>MGSDKIHHHHHHENLYFQGMKQIPQDFRLIEDFFRTRRSVRKFIDRPVEEEKLMAILEAGRIAPSAHNYQPWHFLVVREEEGRKRLAPCSQQPWFPGAPIYIITLGDHQRAWKRGAGDSVDIDTSIAMTYMMLEAHSLGLGCTWVCAFDQALCSEIFDIPSHMTPVS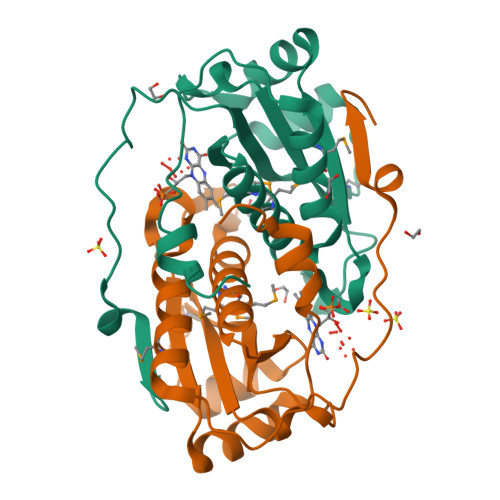ILALGYGDPTVPPREAFNRKTIEEVVSFEKL[2x]> MADLKLPTNLAY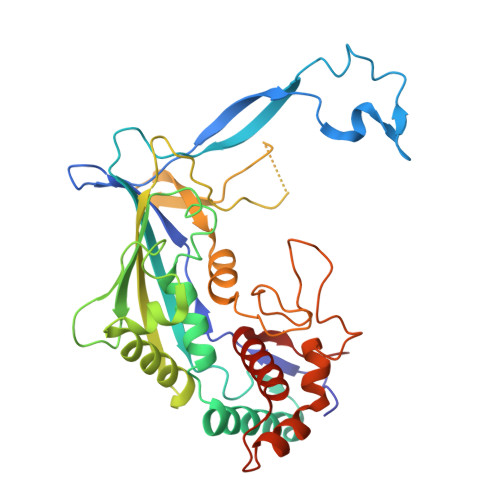ERSIDPSDVCFFVVWPDDRKTPLTYNSRTLLGQMEAASLAYDVSGQPIKSATAEALAQGNPHQVDFCHVPYGASHIECSFSVSFSSELRQPYKCNSSKVKQTLVQLVELYETKIGWTELATRYLMNICNGKWLWKNTRKAYCWNIVLTPWPWNGEKVGFEDIRTNYTSRQDFKNNKNWSAIVEMIKTAFSSTDGLAIFEVRATLHLPTNAMVRPSQVFTEKESGSKSKSKTQNSRVFQSTTIDGERSPILGAFKTGAAIATIDDWYPEATEPLRVGRFGVHREDVTCYRHPSTGKDFFSILQQAEHYIEVLSANKTPAQETINDMHFLMANLIKGGMFQHKGD>[3x]MEVRKVIAAGEVIESPVDVVKELVENSLDAKATKVEVEIVKGGKRLIRVKDNGTGIHPEDVEKVVLQGATSKIETEKDLMNISTYGFRGEALYSISSVSKFKLRSRFFQEKEGKEIEVEAGNILGTRRVGMPVGTEVEVRDLFFNLPVRRKFLKK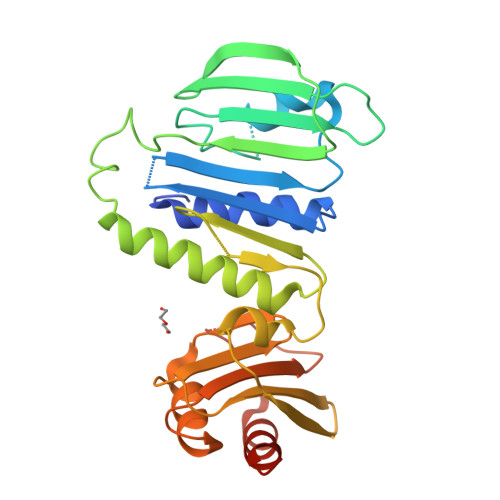EDTERRKVLELIKEYALTNPEVEFTLFSEGRETLKLKKSSLKERVEEVFQTKTEELYAEREGITLRAFVSRNQRQGKYYVFINKRPIQNKNLKEFLRKVFGYKTLVVLYAELPPFMVDFNVHPKKKEVNILKERKFLELVRELAGKEKPIVDI>GHMVSCSAPGKIYLFGEHAVVYGETAIACAVELRTRVRAELNDSITIQSQIGRTGLDFEKHPYVSAVIEKMRKSIPINGVFLTVDSDIPVGSGLGSSAAVTIASIGALNELFGFGLSLQEIAKLGHEIEIKVQGAASPTDTYVSTFGGVVTIPERRKLKTPDCGIVIGDTGVFSSTKELVANVRQLRESYPDLIEPLMTSIGKISRIGEQLVLSGDYASIGRLMNVNQGLLDALGVNILELSQLIYSARAAGAFGAKITGAGGGGCMVALTAPEKCNQVAEAVAGAGGKVTITKPTEQGLKVD[2x]

A key regulatory step in the mevalonate pathway is the ATP-dependent phosphorylation of (R)-mevalonate to (R)-5-phosphomevalonate catalyzed by the enzyme mevalonate kinase (MK), a member of the galacto-/homoserine/mevalonate/phosphomevalonate (GHMP) kinase family. Distributed widely across eukaryotes, bacteria, and archaea, the mevalonate pathway consists of seven enzymes that convert three molecules of acetyl-CoA to isopentenyl pyrophosphate (IPP) and dimethylallyl pyrophosphate (DMAPP), the isomeric, five-carbon precursors to all steroids and isoprenoids. Each MK monomer consists of two domains, where the active site lies on a surface cleft at the interdomain interface. To shed greater light onto the mechanism of MK and to further investigate archaeal MK in particular, we determined the X-ray structures of MmMK bound with the substrate mevalonate and with the product 5-phosphomevalonate.

Mevalonate binds to MmMK at the same location and in a similar position as previously observed in the structure of mevalonate-bound LmMK. However, in both chains of the structure mevalonate makes very few direct contacts with the MmMK protein, in contrast with the several contacts between mevalonate and LmMK. However, many of the contacts observed in the LmMK structure are lost in our mevalonate-bound MmMK structure, where the only direct interaction remaining is between the mevalonate C3-hydroxyl group and His16 (MmMK numbering, corresponding to His25 of LmMK). In fact, the β-strand of LmMK that directly interacts with the mevalonate carboxylate is shortened considerably in MmMK such that there are no residues in this region that can reach mevalonate; in place of the LmMK residue Tyr167 that makes a hydrogen bond with mevalonate, MmMK contains Ile150, which is not capable of interacting with mevalonate. Instead of forming direct interactions with the protein, mevalonate bound to MmMK interacts with several ordered water molecules that themselves form hydrogen bonds to the protein. In this way, water molecules form a cage around the substrate to mediate bridging hydrogen bonding interactions with the protein, including with the backbone amide of Val18 as well as the side chains of Lys9, Ser135, and Asp138. Electron density also indicated that two conformations of mevalonate were present in chain B of the mevalonate-bound structure, and occupancy refinement in Phenix yielded occupancies of ~0.5 for both conformers. These two mevalonate conformations differ only in the position of the carboxylate group, which faces the solvent exterior, indicating that this moiety may “swing” into two different orientations at the protein surface. However, the prior mevalonate-bound LmMK structure as well as our mevalonate-bound MmMK structure presented here suggest that this aspartate residue may be too far from mevalonate to directly deprotonate the C5-hydroxyl, with distances of 5.2 and 5.5 Å, respectively.>ALYEDPPDQKTSPSGKPATLKICSWNVDGLRAWIKKKGLDWVKEEAPDILCLQETKC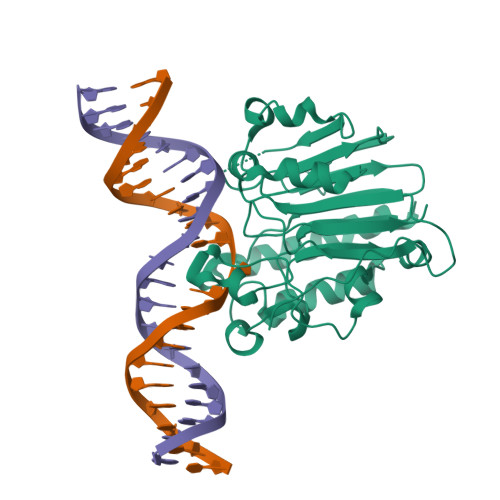SENKLPAELQELPGLSHQYWSAPSDKEGYSGVGLLSRQAPLKVSYGIGDEEHDQEGRVIVAEFDSFVLVTAYVPAAGRGLVRLEYRQRWDEAFRKFLKGLASRKPLVLCGDLNVAHEEIDLRNPKGNKKNAGFTPQERQGFGELLQAVPLADSFRHLYPNTPYAYTFWTYMMNARSKNVGWRLDYFLLSHSLLPALCDSKIRSKALGSDHCPITLYLAL[2x]>MGSYSSDDVEVIREAGRAQGLATILAIGTATP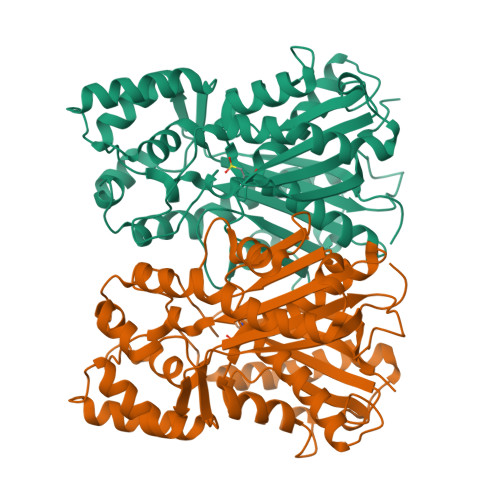PNCVAQADYADYYFRVTKSEHMVDLKEKFKRICEKTAIKKRYLALTEDYLQENPTMCEFMAPSLNARQDLVVTGVPMLGKEAAVKAIDEWGLPKSKITHLIFCTTAGVDMPGADYQLVKLLGLSPSVKRYMLYQQGCAAGGTVLRLAKDLAENNKGSRVLIVCSEITAILFHGPNENHLDSLVAQALFGDGAAALIVGSGPHLAVERPIFEIVSTDQTILPDTEKAMKLHLREGGLTFQLHRDVPLMVAKNIENAAEKALSPLGITDWNSVFWMVHPGGRAILDQVERKLNLKEDKLRASRHVLSEYGNLISACVLFIIDEVRKRSMAEGKSTTGEGLDCGVLFGFGPGMTVETVVLRSVRVTAAVANGN[2x]>[2x]EEKDEEFPEQKAGEVINQPMMMAARQLHDEARKWSSKGNDIIAAAKRMALLMAEMSRLVRGGSGTKRALIQCAKDIAKASDEVTRLAKEVAKQCTDKRIRTNLLQVCERIPTISTQLKILSTVKATMLGRTNISDEESEQATEMLVHNAQNLMQSVKETVREAEAASIKIRTDAGFTLRWVRKTPWYQ;>LDPEEIRKRLEHTERQFRNRRK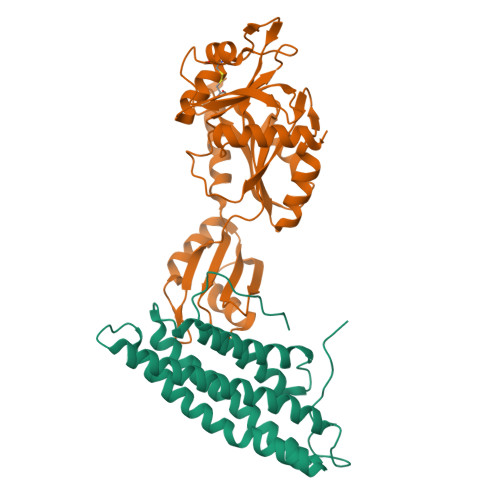ILIRGLPGDVTNQEVHDLLSDYELKYCFVDKYKGTAFVTLLNGEQAEAAINAFHQSRLRERELSVQLQPTDALLCVANLPPSLTQQQFEELVRPFGSLERCFLVYSERTGQSKGYGFAEYMKKDSAARAKSDLLGKPLGPRTLYVHWTDAGQLTPALLHSRCLCVDRLPPGFNDVDALCRALSAVHSPTFCQLACGQDGQLKGFAVLEYETAEMAEEAQQQADGLSLGGSHLRVSFCAPGPPGRSMLAALIAAQATALNRG[2x]>[2x]SNAFRRKLTALDYHNPAGFNCKDETEFR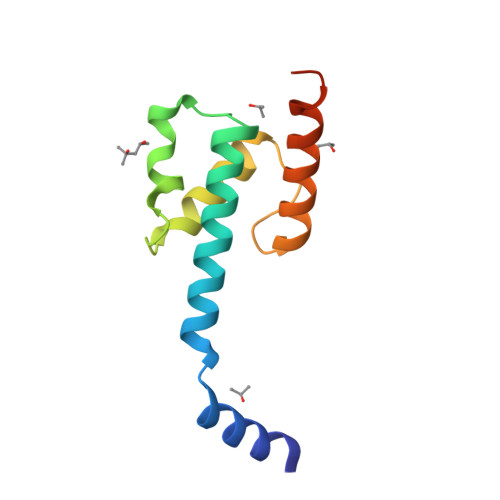NFIVWLEDQKIRHYKIEDRGNLRNIHSSDWPKFFEKYLRDVNCPFKIQDRQEAIDWLLGLAVRLEYGDNAEKYKD>[2x]SHMKFTIQKDRLVESVQDVLKAVSSRTTIPILTGIKIVASDDGVSFTGSD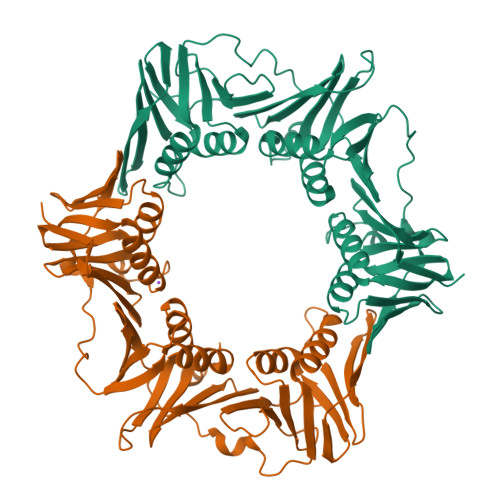SDISIESFIPKEEGDKEIVTIEQPGSIVLQARFFSEIVKKLPMATVEIEVQNQYLTIIRSGKAEFNLNGLDADEYPHLPQIEEHHAIQIPTDLLKNLIRQTVFAVSTSETRPILTGVNWKVEQSELLCTATDSHRLALRKAKLDIPEDRSYNVVIPGKSLTELSKILDDNQELVDIVITETQVLFKAKNVLFFSRLLDGNYPDTTSLIPQDSKTEIIVNTKEFLQAIDRASLLAREGRNNVVKLSAKPAESIEISSNSPEIGKVVEAIVADQIEGEELNISFSPKYMLDALKVLEGAEIRVSFTGAMRPFLIRTPNDETIVQLILPVRTY> ENLTPQHMASMALTGTDRVKRGMAEMQKGGVIMDVVNAEQAKIAEAAGAVAVMALERVPADIRAAGGVAR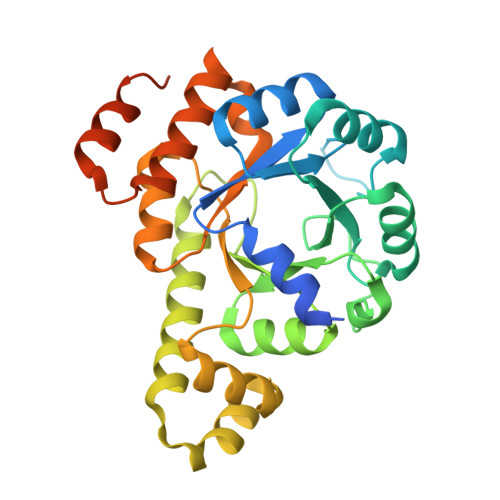MADPTVIEEVMNAVSIPVMAKVRIGHYVEARVLEALGVDYIDESEVLTPADEEFHIDKRQFTVPFVCGCRDLGEAARRIAEGASMLRTKGEPGTGNIVEAVRHMRKVNAQIRKVVNMSEDELVAEAKQLGAPVEVLREIKRLGRLPVVNFAAGGVTTPADAALMMHLGADGVFVGSGIFKSENPEKYARAIVEATTHYEDYELIAHLSKGLGGAMRGIDIATLLPEHRMQERGWA>MKLVAQGSTLDL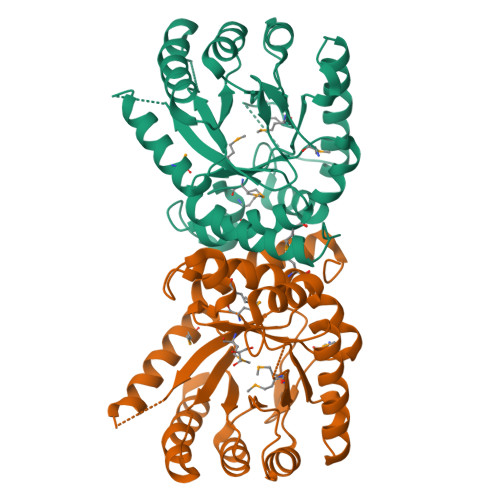SHPHVMGILNVTPDSFSDGGAHNSLIEAVKHANLMINAGATIIDIGGESTRPGAAEVSVEEELARVIPVVEAIAQRFEVWISVDTSKAEVIRQSARAGAHIINDIRSLTEPGALQAAAETGLPVCLMHMQGQPKTMQEAPKYEDVFADVERFFNEHIVRCEQAGIAKEKLLLDPGFGFGKNLSHNYQLLARLGEFHHFGLPLLVGMSRKSMVGQLLNVGPSERLNGSLACAVIAAMQGAQIIRVHDVKETVEALRVVEATLAAKGKKRYE[2x]> GSEGHRTLASTPALWASIPCPRSELRLDLVLPSGQSFRWREQSPAHWSGVLADQVWTLTQTEEQLHCTVYRGDKSQASRPTPDELEAVRKYFQLDVTLAQLYHHWGS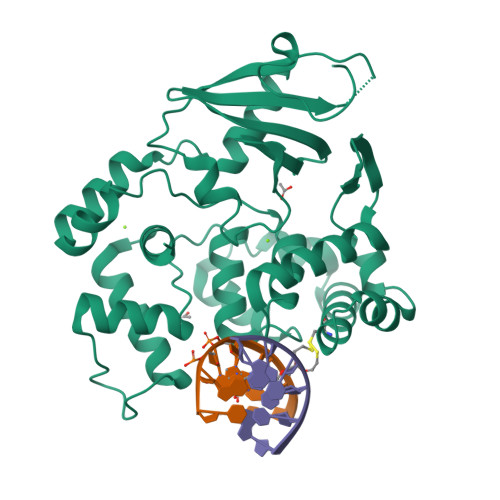VDSHFQQVAQKFQGVRLLRQDPIECLFSFICSSNNNIARITGMVERLCQAFGPRLIQLDDVTYHGFPSLQALAGPEVEAHLRKLGLGYRARCVSASARAILEEQGGLAWLQQLRESSYEEAHKALCILPGVGTKVADWICLMALDKPQAVPVDVHMWHIAQRDYSWHPTTSQAKGPSPQTNKELGNFFRSLWGPYAGWAQAVLFSADLRQ>[4x]CPPKCRCEKLLFYCDSQGFHSVPNATDKGSLGLSLRHNHITELERDQFASFSQLTWLHLDHNQISTVKEDAFQGLYKLKELILSSNKIFYLPNTTFTQLINLQNLDLSFNQLSSLHPELFYGLRKLQTLHLRSNSLRTIPVRLFWDCRSLEFLDLSTNRLRSLARNGFAGLIKLRELHLEHNQLTKINFAHFLRLSSLHTLFLQWNKISNLTCGMEWTWGTLEKLDLTGNEIKAIDLTVFETMPNLKILLMDNNKLNSLDSKILNSLRSLTTVGLSGNLWECSARICALASWLGSFQGRWEHSI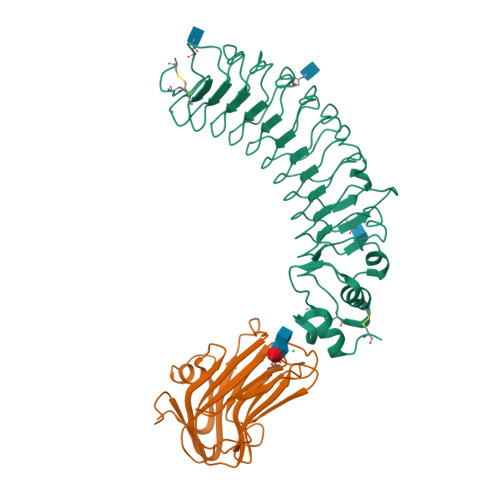LCHSPDHTQGEDILDAVAGFQLCWNLSTTVTVMAGSHHHHHH;>DAASHAGTTYIFSKGGGQITYKWPPNDRPSTRADRLAIGFSTVQKEAVLVRVDSSSGLGDYLELHIHQGKIGVKFNVGTDDIAIEESNAIINDGKYHVVRFTRSGGNATLQVDSWPVIERYPAGRQLTIFNSQATIIIGGKEQGQPFQGQLSGLYYNGLKVLNMAAENDANIAIVGNVRLVGEVPGSHHHHHH[4x]> MRGSHHHHHHTDPTGATFPEEAIADLSVNMYNRLRATGEDENILFSPLSIALAMGMMELGAQGSTQKEIRHSMGYDSLKNGEEFSFLKEFSNMVTAKESQYVMKIANSLFVQNGFHVNEEFLQMMKKYFNAAVNHVDFSQNVAVANYINKWVENNTNNLVKDLVSPRDFDAATYLALINAVYFKGNWKSQFRPENTRTFSFTKDDESEVQIPMMYQQGEFYYGEFSDGSNEAGGIYQVLEIPYEGDEISMMLVLSRQEVPLATLEPLVKAQL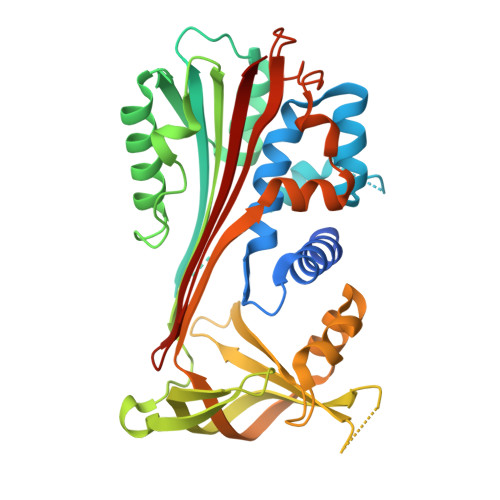VEEWANSVKKQKVEVYLPRFTVEQEIDLKDVLKALGITEIFIKDANLTGLSDNKEIFLSKAIHKSFLEVNEEGSEAAAVSGMIAISR> MKHHHHHHPMANGAELIIQEINKEAERKIEYILNEARQQAEKIKEEARRNAEAKAEWIIRRAKTQAELEKQRIIANARLEVRRKRLAIQEEIISSVLEEVKRR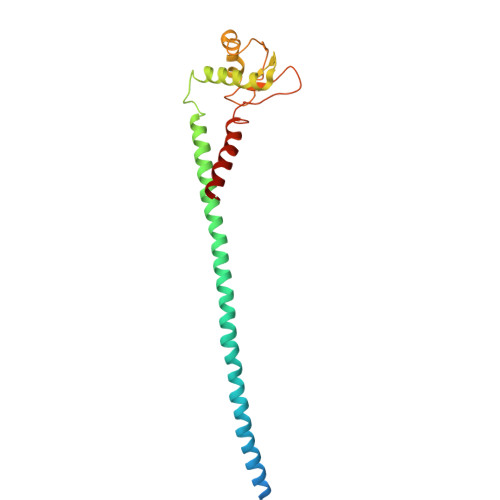LETMSEDEYFESVKALLKEAIKELNEKKVRVMSNEKTLGLIASRIEEIKSELGDVSIELGETVDTMGGVIVETEDGRIRIDNTFEARMERFEGEIRSTIAKVLFG> HMASMKKKGSVVIVGRINLSGDTAYAQQTRGEEGCQETSQTGRDKNQVEGEVQIVSTATQTFLATSINGVLWTVYHGAGTRTIASPKGPVTQMYTNVDKDLVGWQAPQGSRSLTPCTCGSSDL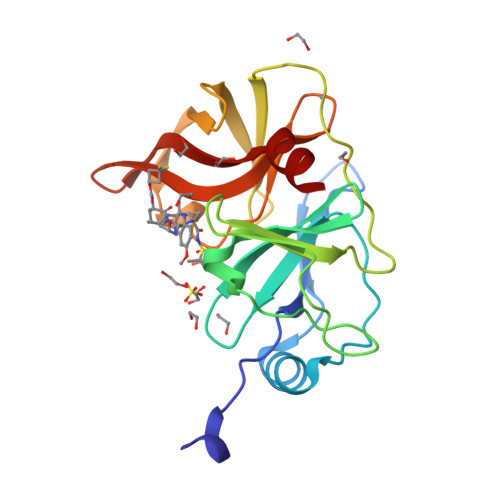YLVTRHADVIPVRRRGDSRGSLLSPRPISYLKGSSGGPLLCPAGHAVGIFRAAVSTRGVAKAVAFIPVESLETTM>[2x]KESAAAKFERQHMDSGNSPSSSSNYCNLMMCCRKMTQGKCK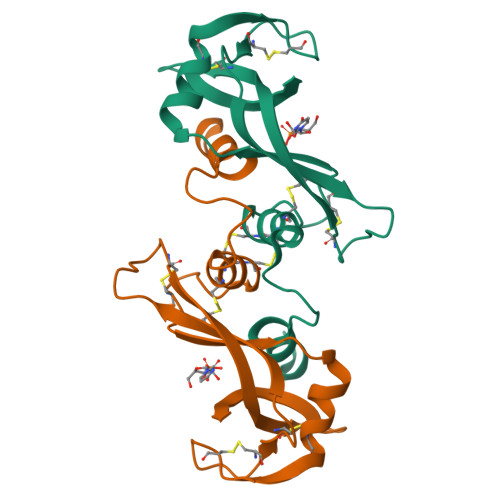PVNTFVHESLADVKAVCSQKKVTCKNGQTNCYQSKSTMRITDCRETGSSKYPNCAYKTTQVEKHIIVACGGKPSVPVHFDASV Here, we demonstrate that the centriolar protein SAS-6 forms rod-shaped homodimers that interact through their N-terminal domains to form oligomers. Proteins of the SAS-6 family comprise an N-terminal domain with the evolutionarily conserved PISA motif, followed by a segment with a predicted coiled coil and a less-conserved C-terminal region predicted to be disordered. Furthermore and in conclusion, because these residues are well conserved among SAS-6 orthologs, we propose that the self-assembly of SAS-6 homodimers into a 9-fold symmetric ring structure is a fundamental property at the root of the universal 9-fold symmetry of centrioles.

To investigate the structural organization of the Bld12p N-terminal domains in the context of the two-stranded parallel coiled coil, we produced a fragment in which the crN variant was extended by the first six heptad repeats of the Bld12p coiled coil (crN-6HR). AUC experiments conducted at 150 μM protein concentration revealed that crN-6HR forms higher-order oligomeric species. However, a mutant in which F145 was substituted for glutamate (crN-6HR[F145E]) formed only dimers, as revealed by AUC and MALS experiments. We solved the structure of Bld12p crN-6HR[F145E] to 3.0 Å resolution by X-ray crystallography. The asymmetric unit of the crystal revealed a dimer (denoted the crCC-dimer hereafter). Dimerization is brought about by interactions between the two α3 helices, which establish a parallel, two-stranded coiled coil through knobs-into-hole packing of the residues occupying the heptad a and d core positions. The relative orientation of the two N-terminal domains is maintained by predominantly hydrophobic interactions formed between residues of their β3-β4 loops and residues from both coiled-coil α3 helices. Having the structures of both the crN-dimer and the crCC-dimer of Bld12p allowed us to build a structural model of higher-order oligomers using both dimer interfaces. Strikingly, when crCC-dimers were associated such that their N-terminal domains interact as observed in the crN-dimer, we obtained a ring with a 9-fold symmetry (see Experimental Procedures for full description of the modeling). In this structural model, the long axes of the coiled-coil domains are in plane with and radiate out from the ring, which is ∼3.5 × 5 nm in thickness and ∼23 nm in mean diameter.

>GSMPLLLDDGDPKAQTGFDLSTATTLFWRPVPVHVKQQDREDVLEELTFRILTGVAKQNHNLRILRIHISSDSDLFFLHTLEVSEEDFQSLKNDQGILVDFASFPGKIISLLEKCILAQPGDSPRFQAVLTIRGGESVFKIVEINDEKQLPHITLAFRPGNDSVVKQFLAFRLSEVKGTCHDLSDDLSRTRDDRDSMVAQLAQCRQQLAQLREQYDKHLLEVQAQAKT[2x]>MTKQYKNYVNGEWKLSENEIKIYEPASGAELGSVPAMSTEEVDYVYASAKKAQPAWRALSYIERAAYLHKVADILMRDKEKIGAILSKEVAKGYKSAVSEVVRTAEIINYAAEEGLRMEGEVLEGGSFEAASKKKIAVVRREPVGLVLAISPFNYPVNLAGSKIAPALIAGNVIAFKPPTQGSISGLLLAEAFAEAGLPAGVFNTITGRGSEIGDYIVEHQAVNFINFTGSTGIGERIGKMAGMRPIMLALGGKDSAIVLE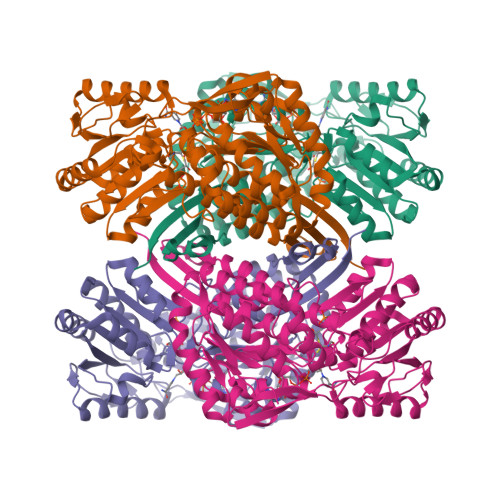DADLELTAKNIIAGAFGYSGQRCTAVKRVLVMESVADELVEKIREKVLALTIGNPEDDADITPLIDTKSADYVEGLINDANDKGATALTEIKREGNLICPILFDKVTTDMRLAWEEPFGPVLPIIRVTSVEEAIEISNKSEYGLQASIFTNDFPRAFGIAEQLEVGTVHINNKTQRGTDNFPFLGAKKSGAGIQGVKYSIEAMTTVKSVVFDIK[4x]> LTAKHRPSVVWLHNAECDGCTEAAIRTIKPYIDALILDTISLDYQETIMAAAGEAAEAALHQALEGKDGYYLVVEGGLPTIDGGQWGMVAGHPMIETTKKAAAKAKGIICIGTCSAYGGVQKAKPN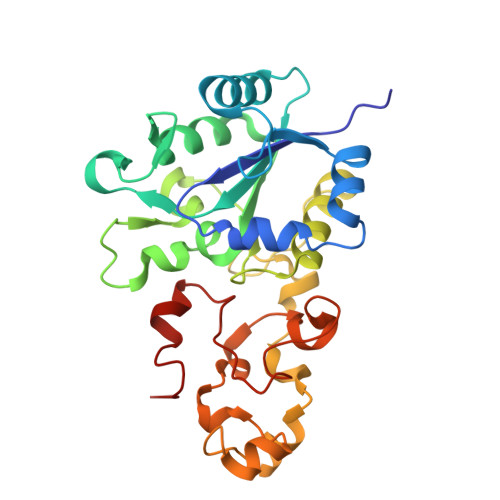PSQAKGVSEALGVKTINIPGCPPNPINFVGAVVHVLTKGIPDLDENGRPKLFYGELVHDNCPRLPHFEASEFAPSFDSEEAKKGFCLYELGCKGPVTYNNCPKVLFNQVNWPVQAGHPCLGCSEPDFWDTMTPFYEQG> MSVIDSILDKADEQEIKKLNVIVDKIDALEDSMKNLSYEELKDMTAIFKNRLKKGETLDDILPEAFAVVREVSKRKLGMRQYRVQLIGGIVIHQGKIAEMKTGEGKTLVEVAPVYLNALTGKGVHVITVNDYLAERDKELMSPVYESLGMTVGVIISNQDPNIRKQQYKCDITYGTNSEFGFDYLRDNMVPDLSHKVQRELNFAIVDEVDSILIDEARTPLIIAGDGDEDLKLYELANSFVKTVKEEDFELDRKDKTIALTASGISKAESFFGITNLTDIKNIELYHHINQALRGHKLMEKDVDYVISNGEVMIVDEFTGRVMDGRRYTDGLHQAIEAKEGVEIKNESKTMATVTYQNFFRLYEKLSGMTGTAKTEEGEFESIYKLNVVQIPTNRPVIRADLHDKVFKTEEEKYSAVVEEIIRIHKTRQPILVGTVSVEKSEKLSKML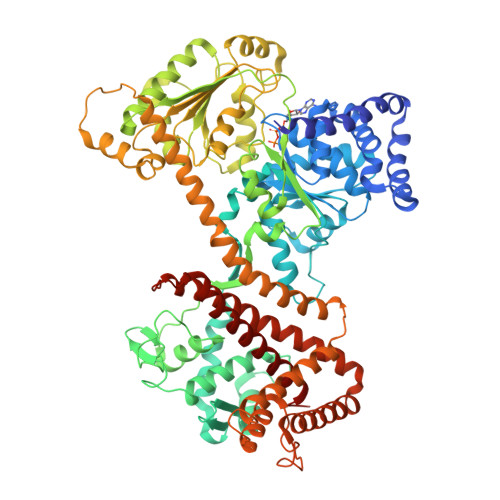KKQGIKHQVLNAKQHDKEAEIISKAGKLDAITIATNMAGRGTDISLGAGDKEEEQEVKDLGGLYVIGTERHESRRIDNQLRGRSGRQGDPGTSRFFVSLEDDVIKLYGGKTIEKLMKRTSSNENTAIESKALTRAIERAQKGVEGKNFEIRKNVLKYDDTINEQRKVIYNERNKVLNDEDIQEDIQKMVKDIIQEAGETYLIGRKRDYYGYFKHLYSTFMPADTLLIPGVDKKSVQEIIDSTYEISKRVYDLKKMMLGIDKVAELEKTVLLKVVDQYWIDHIDAMEQLKQYIGLKSYAQKDPFKEYALEGYDMFEALNKNIREATVQYLYKFN>GGEIRPTIGQQMETGDQRFGDLVFRQLAPNVWQHTSYLDMPGFGAVASNGLIVRDGGRVLVVDTAWTDDQTAQILNWIKQEINLPVALAVVTHAHQDKMGGMDALHAAGIATYANALSNQLAPQEGMVAAQHSLTFAANGWVEPATAPNFGPLKVFYPGPGHTSDNITVGIDGTDIAFGGCLIKDSKAKSLG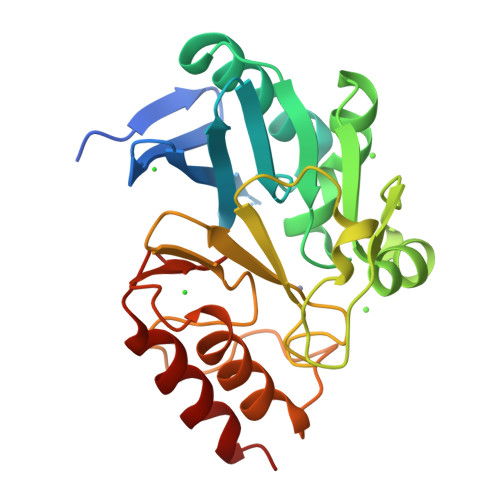NLGDADTEHYAASARAFGAAFPKASMIVMSHSAPDSRAAITHTARMADKLR[2x]> GSGRMSGGSSCSQTPSRAIPATRRVVLGDGVQLPPGDYSTTPGGTLFSTTPGGTRIIYDRKFLMECRNSPVTKTPPRDLPTIPGVTSPSSDEP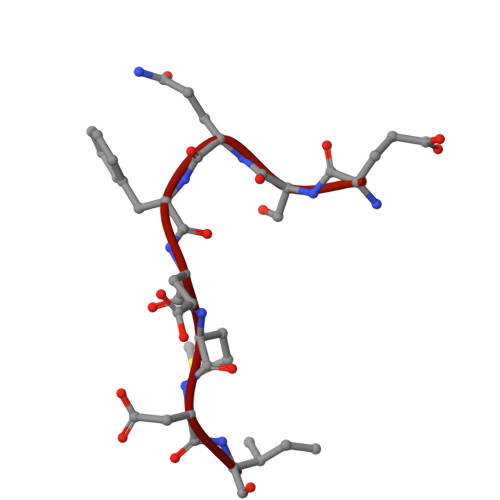PMEASQSHLRNSPEDKRAGGEESQFEMDI> MHHGTGPQNVQHQLQRSRACPGSEGEEQPAHPNPPPSPAAPFAPSASPSAPQSPSYQIQQLMNRSPATGQNVNITLQSVGPVVGGNQQITLAPLPLPSPTSPGFQFSAQPRRFEHGSPSYIQVTSPLSQQVQTQSPTQPSPGPGQALQNVRAGAPGPGLGLCSSSPTGGFVDASVLVRQISLSPSSGGHFVFQDGSGLTQIAQGAQVQLQHPGTPITVRERRPSQPHTQSGGTIHHLGPQSPAAAGGAGLQPLASPSHITTANLPPQISSIIQGQLVQQQQVLQGPPLPRPLGFERTPGVLLPGAGGAAGFGMTSPPPPTSPSRTAVPPGLSSLPLTSVGNTGMKKVPKKLEEIPPASPEMAQMRKQCLDYHYQEMQALKEVFKEYLIELFFLQHFQGNMMDFLAFKKKHYAPLQAYLRQNDLDIEEEEEEEEEEEEKSEVINDEVKVVTGKDGQTGTPVAIATQLPPKVSAAFSSQQQPFQQALAGSLVAGAGSTVETDLFKRQQAMPSTGMAEQSKRPRLEVGHQGVVFQHPGADAGVPLQQLMPTAQGGMPPTPQAAQLAGQRQSQQQYDPSTGPPVQNAASLHTPLPQLPGRLPPAGVPTAALSSALQFAQQPQVVEAQTQLQIPVKTQQPNVPIPAPPSSQLPIPPSQPAQLALHVPTPGKVQVQASQLSSLPQMVASTRLPVDPAPPCPRPLPTSSTSSLAPVSGSGPGPSPARSSPVNRPSSATNKALSPVTSRTPGVVASAPTKPQSPAQNATSSQDSSQDTLTEQITLENQVHQRIAELRKAGLWSQRRLPKLQEAPRPKSHWDYLLEEMQWMATDFAQERRWKVAAAKKLVRTVVRHHEEKQLREERGKKEEQSRLRRIAASTAREIECFWSNIEQVVEIKLRVELEEKRKKALNLQKVSRRGKELRPKGFDALQESSLDSGMSGRKRKASISLTDDEVDDEEETIEEEEANEGVVDHQTELSNLAKEAELPLLDLMKLYEGAFLPSSQWPRPKPDGEDTSGEEDADDCPGDRESRKDLVLIDSLFIMDQFKAAERMNIGKPNAKDIADVTAVAEAILPKGSARVTTSVKFNAPSLLYGALRDYQKIGLDWLAKLYRKNLNGILADEAGLGKTVQIIAFFAHLACNEGNWGPHLVVVRSCNILKWELELKRWCPGLKILSYIGSHRELKAKRQEWAEPNSFHVCITSYTQFFRGLTAFTRVRWKCLVIDEMQRVKGMTERHWEAVFTLQSQQRLLLIDSPLHNTFLELWTMVHFLVPGISRPYLSSPLRAPSEESQDYYHKVVIRLHRVTQPFILRRTKRDVEKQLTKKYEHVLKCRLSNRQKALYEDVILQPGTQEALKSGHFVNVLSILVRLQRICNHPGLVEPRHPGSSYVAGPLEYPSASLILKALERDFWKEADLSMFDLIGLENKITRHEAELLSKKKIPRKLMEEISTSAAPAARPAAAKLKASRLFQPVQYGQKPEGRTVAFPSTHPPRTAAPTTASAAPQGPLRGRPPIATFSANPEAKAAAAPFQTSQASASAPRHQPASASSTAASPAHPAKLRAQTTAQASTPGQPPPQPQAPSHAAGQSALPQRLVLPSQAQARLPSGEVVKIAQLASITGPQSRVAQPETPVTLQFQGSKFTLSHSQLRQLTAGQPLQLQGSVLQIVSAPGQPYLRAPGPVVMQTVSQAGAVHGALGSKPPAGGPSPAPLTPQVGVPGRVAVNALAVGEPGTASKPASPIGGPTQEEKTRLLKERLDQIYLVNERRCSQAPVYGRDLLRICALPSHGRVQWRGSLDGRRGKEAGPAHSYTSSSESPSELMLTLCRCGESLQDVIDRVAFVIPPVVAAPPSLRVPRPPPLYSHRMRILRQGLREHAAPYFQQLRQTTAPRLLQFPELRLVQFDSGKLEALAILLQKLKSEGRRVLILSQMILMLDILEMFLNFHYLTYVRIDENASSEQRQELMRSFNRDRRIFCAILSTHSRTTGINLVEADTVVFYDNDLNPVMDAKAQEWCDRIGRCKDIHIYRLVSGNSIEEKLLKNGTKDLIREVAAQGNDYSMAFLTQRTIQELFEVYSPMDDAGFPVKAEEFVVLSQEPSVTETIAPKIARPFIEALKSIEYLEEDAQKSAQEGVLGPHTDALSSDSENMPCDEEPSQLEELADFMEQLTPIEKYALNYLELFHTSIEQEKERNSEDAVMTAVRAWEFWNLKTLQEREARLRLEQEEAELLTYTREDAYSMEYVYEDVDGQTEVMPLWTPPTPPQDDSDIYLDSVMCLMYEATPIPEAKLPPVYVRKERKRHKTDPSAAGRKKKQRHGEAVVPPRSLFDRATPGLLKIRREGKEQKKNILLKQQVPFAKPLPTFAKPTAEPGQDNPEWLISEDWALLQAVKQLLELPLNLTIVSPAHTPNWDLVSDVVNSCSRIYRSSKQCRNRYENVIIPREEGKSKNNRPLRTSQIYAQDENATHTQLYTSHFDLMKMTAGKRSPPIKPLLGMNPFQKNPKHASVLAESGINYDKPLPPIQVASLRAERIAKEKKALADQQKAQQPAVAQPPPPQPQPPPPPQQPPPPLPQPQAAGSQPPAGPPAVQPQPQPQPQTQPQPVQAPAKAQPAITTGGSAAVLAGTIKTSVTGTSMPTGAVSGNVIVNTIAGVPAATFQSINKRLASPVAPGALTTPGGSAPAQVVHTQPPPRAVGSPATATPDLVSMATTQGVRAVTSVTASAVVTTNLTPVQTPARSLVPQVSQATGVQLPGKTITPAHFQLLRQQQQQQQQQQQQQQQQQQQQQQQQQQQQQTTTTSQVQVPQIQGQAQSPAQIKAVGKLTPEHLIKMQKQKLQMPPQPPPPQAQSAPPQPTAQVQVQTSQPPQQQSPQLTTVTAPRPGALLTGTTVANLQVARLTRVPTSQLQAQGQMQTQAPQPAQVALAKPPVVSVPAAVVSSPGVTTLPMNVAGISVAIGQPQKAAGQTVVAQPVHMQQLLKLKQQAVQQQKAIQPQAAQGPAAVQQKITAQQITTPGAQQKVAYAAQPALKTQFLTTPISQAQKLAGAQQVQTQIQVAKLPQVVQQQTPVASIQQVASASQQASPQTVALTQATAAGQQVQMIPAVTATAQVVQQKLIQQQVVTTASAPLQTPGAPNPAQVPASSDSPSQQPKLQMRVPAVRLKTPTKPPCQ;> MAFVATQGATVVDQTTLMKKYLQFVAALTDVNTPDETKLKMMQEVSENFENVTSSPQYSTFLEHIIPRFLTFLQDGEVQFLQEKPAQQLRKLVLEIIHRIPTNEHLRPHTKNVLSVMFRFLETENEENVLICLRIIIELHKQFRPPITQEIHHFLDFVKQIYKELPKVVNRYFENPQVIPENTVPPPEMVGMITTIAVKVNPEREDSETRTHSIIPRGSLSLKVLAELPIIVVLMYQLYKLNIHNVVAEFVPLIMNTIAIQVSAQARQHKLYNKELYADFIAAQIKTLSFLAYIIRIYQELVTKYSQQMVKGMLQLLSNCPAETAHLRKELLIAAKHILTTELRNQFIPCMDKLFDESILIGSGYTARETLRPLAYSTLADLVHHVRQHLPLSDLSLAVQLFAKNIDDESLPSSIQTMSCKLLLNLVDCIRSKSEQESGNGRDVLMRMLEVFVLKFHTIARYQLSAIFKKCKPQSELGAVEAALPGVPTAPAAPGPAPSPAPVPAPPPPPPPPPPATPVTPAPVPPFEKQGEKDKEDKQTFQVTDCRSLVKTLVCGVKTITWGITSCKAPGEAQFIPNKQLQPKETQIYIKLVKYAMQALDIYQVQIAGNGQTYIRVANCQTVRMKEEKEVLEHFAGVFTMMNPLTFKEIFQTTVPYMVERISKNYALQIVANSFLANPTTSALFATILVEYLLDRLPEMGSNVELSNLYLKLFKLVFGSVSLFAAENEQMLKPHLHKIVNSSMELAQTAKEPYNYFLLLRALFRSIGGGSHDLLYQEFLPLLPNLLQGLNMLQSGLHKQHMKDLFVELCLTVPVRLSSLLPYLPMLMDPLVSALNGSQTLVSQGLRTLELCVDNLQPDFLYDHIQPVRAELMQALWRTLRNPADSISHVAYRVLGKFGGSNRKMLKESQKLHYVVTEVQGPSITVEFSDCKASLQLPMEKAIETALDCLKSANTEPYYRRQAWEVIKCFLVAMMSLEDNKHALYQLLAHPNFTEKTIPNVIISHRYKAQDTPARKTFEQALTGAFMSAVIKDLRPSALPFVASLIRHYTMVAVAQQCGPFLLPCYQVGSQPSTAMFHSEENGSKGMDPLVLIDAIAICMAYEEKELCKIGEVALAVIFDVASIILGSKERACQLPLFSYIVERLCACCYEQAWYAKLGGVVSIKFLMERLPLTWVLQNQQTFLKALLFVMMDLTGEVSNGAVAMAKTTLEQLLMRCATPLKDEERAEEIVAAQEKSFHHVTHDLVREVTSPNSTVRKQAMHSLQVLAQVTGKSVTVIMEPHKEVLQDMVPPKKHLLRHQPANAQIGLMEGNTFCTTLQPRLFTMDLNVVEHKVFYTELLNLCEAEDSALTKLPCYKSLPSLVPLRIAALNALAACNYLPQSREKIIAALFKALNSTNSELQEAGEACMRKFLEGATIEVDQIHTHMRPLLMMLGDYRSLTLNVVNRLTSVTRLFPNSFNDKFCDQMMQHLRKWMEVVVITHKGGQRSDGNESISECGRCPLSPFCQFEEMKICSAIINLFHLIPAAPQTLVKPLLEVVMKTERAMLIEAGSPFREPLIKFLTRHPSQTVELFMMEATLNDPQWSRMFMSFLKHKDARPLRDVLAANPNRFITLLLPGGAQTAVRPGSPSTSTMRLDLQFQAIKIISIIVKNDDSWLASQHSLVSQLRRVWVSENFQERHRKENMAATNWKEPKLLAYCLLNYCKRNYGDIELLFQLLRAFTGRFLCNMTFLKEYMEEEIPKNYSIAQKRALFFRFVDFNDPNFGDELKAKVLQHILNPAFLYSFEKGEGEQLLGPPNPEGDNPESITSVFITKVLDPEKQADMLDSLRIYLLQYATLLVEHAPHHIHDNNKNRNSKLRRLMTFAWPCLLSKACVDPACKYSGHLLLAHIIAKFAIHKKIVLQVFHSLLKAHAMEARAIVRQAMAILTPAVPARMEDGHQMLTHWTRKIIVEEGHTVPQLVHILHLIVQHFKVYYPVRHHLVQHMVSAMQRLGFTPSVTIEQRRLAVDLSEVVIKWELQRIKDQQPDSDMDPNSSGEGVNSVSSSIKRGLSVDSAQEVKRFRTATGAISAVFGRSQSLPGADSLLAKPIDKQHTDTVVNFLIRVACQVNDNTNTAGSPGEVLSRRCVNLLKTALRPDMWPKSELKLQWFDKLLMTVEQPNQVNYGNICTGLEVLSFLLTVLQSPAILSSFKPLQRGIAACMTCGNTKVLRAVHSLLSRLMSIFPTEPSTSSVASKYEELECLYAAVGKVIYEGLTNYEKATNANPSQLFGTLMILKSACSNNPSYIDRLISVFMRSLQKMVREHLNPQAASGSTEATSGTSELVMLSLELVKTRLAVMSMEMRKNFIQAILTSLIEKSPDAKILRAVVKIVEEWVKNNSPMAANQTPTLREKSILLVKMMTYIEKRFPEDLELNAQFLDLVNYVYRDETLSGSELTAKLEPAFLSGLRCAQPLIRAKFFEVFDNSMKRRVYERLLYVTCSQNWEAMGNHFWIKQCIELLLAVCEKSTPIGTSCQGAMLPSITNVINLADSHDRAAFAMVTHVKQEPRERENSESKEEDVEIDIELAPGDQTSTPKTKELSEKDIGNQLHMLTNRHDKFLDTLREVKTGALLSAFVQLCHISTTLAEKTWVQLFPRLWKILSDRQQHALAGEISPFLCSGSHQVQRDCQPSALNCFVEAMSQCVPPIPIRPCVLKYLGK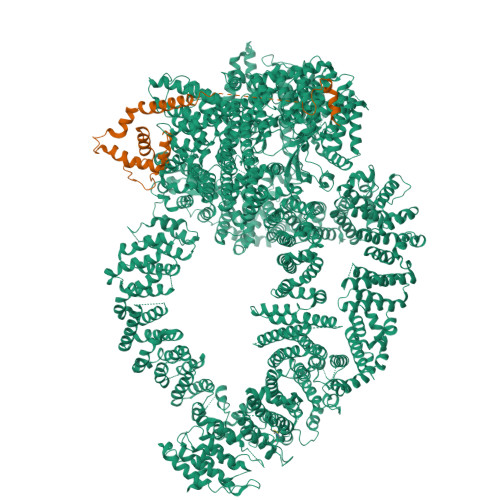THNLWFRSTLMLEHQAFEKGLSLQIKPKQTTEFYEQESITPPQQEILDSLAELYSLLQEEDMWAGLWQKRCKYSETATAIAYEQHGFFEQAQESYEKAMDKAKKEHERSNASPAIFPEYQLWEDHWIRCSKELNQWEALTEYGQSKGHINPYLVLECAWRVSNWTAMKEALVQVEVSCPKEMAWKVNMYRGYLAICHPEEQQLSFIERLVEMASSLAIREWRRLPHVVSHVHTPLLQAAQQIIELQEAAQINAGLQPTNLGRNNSLHDMKTVVKTWRNRLPIVSDDLSHWSSIFMWRQHHYQGKPTWSGMHSSSIVTAYENSSQHDPSSNNAMLGVHASASAIIQYGKIARKQGLVNVALDILSRIHTIPTVPIVDCFQKIRQQVKCYLQLAGVMGKNECMQGLEVIESTNLKYFTKEMTAEFYALKGMFLAQINKSEEANKAFSAAVQMHDVLVKAWAMWGDYLENIFVKERQLHLGVSAITCYLHACRHQNESKSRKYLAKVLWLLSFDDDKNTLADAVDKYCIGVPPIQWLAWIPQLLTCLVGSEGKLLLNLISQVGRVYPQAVYFPIRTLYLTLKIEQRERYKSDPGPIRATAPMWRCSRIMHMQRELHPTLLSSLEGIVDQMVWFRENWHEEVLRQLQQGLAKCYSVAFEKSGAVSDAKITPHTLNFVKKLVSTFGVGLENVSNVSTMFSSAASESLARRAQATAQDPVFQKLKGQFTTDFDFSVPGSMKLHNLISKLKKWIKILEAKTKQLPKFFLIEEKCRFLSNFSAQTAEVEIPGEFLMPKPTHYYIKIARFMPRVEIVQKHNTAARRLYIRGHNGKIYPYLVMNDACLTESRREERVLQLLRLLNPCLEKRKETTKRHLFFTVPRVVAVSPQMRLVEDNPSSLSLVEIYKQRCAKKGIEHDNPISRYYDRLATVQARGTQASHQVLRDILKEVQSNMVPRSMLKEWALHTFPNATDYWTFRKMFTIQLALIGFAEFVLHLNRLNPEMLQIAQDTGKLNVAYFRFDINDATGDLDANRPVPFRLTPNISEFLTTIGVSGPLTASMIAVARCFAQPNFKVDGILKTVLRDEIIAWHKKTQEDTSSPLSAAGQPENMDSQQLVSLVQKAVTAIMTRLHNLAQFEGGESKVNTLVAAANSLDNLCRMDPAWHPWL Recently, the nuclear protein TbPar42 (molecular mass of 42 kDa) has been identified, of which RNAi-induced knockdown in procyclic cells of T. brucei inhibits proliferation of the parasite, suggesting a key role of the protein in cell growth. Protein sequence alignment identified TbPar42 as a two-domain protein, exhibiting an N-terminal flanked forkhead association (FHA) domain and a putative peptidyl-prolyl-cis/trans-isomerase (PPIase) domain connected by a linker region. FHA domains are generally known as phosphopeptide recognition modules, although the TbPar42 FHA domain has not yet been proven to have affinity to phosphorylated substrates. Peptidyl-prolyl cis/trans isomerases are enzymes that accelerate the adjustment of the equilibrium of Xaa–Pro (Xaa being any amino acid) moieties within substrates.

The PPIase adopts a globular fold, which is characteristic for parvulin type proteins. The central β-sheet, composed of four antiparallel β-strands (β3-β4-β1-β2), is surrounded by four α-helices. A comparison of both structures indicates that well-conserved residues of Pin1-like parvulins, e.g., the histidine motif (His59 and His157 in hPin1; His271 and His377 in TbPar42), as well as a characteristic cysteine within the catalytic cleft (Cys113 in hPin1; Cys333 in TbPar42), are located at the same spatial positions within both folds. The hPin1 Ser154, described as a part of the catalytic tetrad is replaced by Leu374 in TbPar42. Residues Leu122, Met130, and Phe134 of Pin1, which are located at the concave side of the β-sheet core, constitute a hydrophobic binding pocket for the substrate’s proline ring moiety. At the same spatial positions, Leu342 and Phe354 can be found in the TbPar42-PPIase structure, whereas the methionine is exchanged by a tyrosine (Tyr350), Figure 3D. A homologous loop is also present in the structure of TbPar42-PPIase. Although the PPIase domain of TbPar42 adopts a parvulin fold and reflects structural elements of Pin1-type proteins, it is catalytically inactive. From all the current data, we may conclude that the PPIase domain of TbPar42 seems to have no enzymatic function within the protein. Residues affected by peptide addition were in near proximity to the proposed proline binding site (Thr265, Gly334, Val345, Thr349, Glu352, Gly353, Phe359 Glu373), but KD values were in the millimolar range (~10 mM). Thus, the structural reason for the absence of activity remains unknown.

> GPPTERHFYHVLVKHKDVRRPSSLAPRNKGEKITRSRADAINLAQAILAQHKERKTWSLDEFVQVVRDFSECGSAKRDGDLGMVESGTYTEGFDTVAFSLKSGEVSAPVETELGVHLIYRVE> SKPRNQQQVCPLQNVPAWGYSLYKGIDMSVPLAYDPNNELGDLKDVFPSAVDEMAIGYVCGNPAVKHVLTWKTTDAIQKPIANGDDWGGVIPVGMPCYSKSIRTTRISATENRETEVMDAAPCEYVANMFSYWRATMCYRITVVKTAFHTGRLEIFFEPGVIPVKPTVNN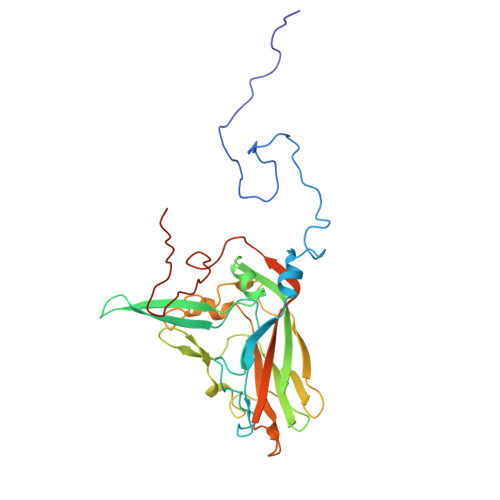IGPDQDRLTGAVAPSDNNYKYILDLTNDTEVTIRVPFVSNKMFLKTAGIYGANSENNWNFHESFSGFLCIRPVTKLMAPDTVSDNVSIVVWKWAEDVVVVEPKPLTSGPTQVYRPPPTASTAVEVLNVEL>GAMGHKIDTKEDMKILYSEI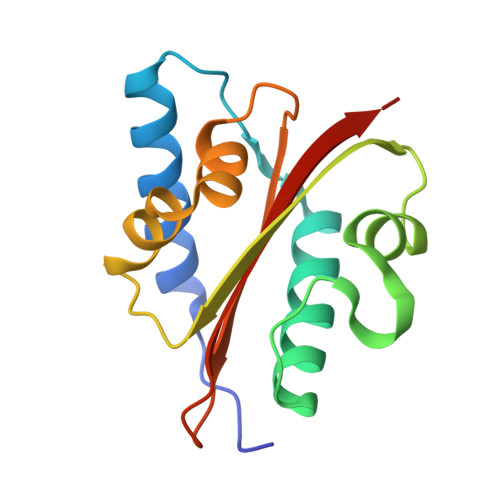AELRKKLNLNHLEIDDTLEKVAKEYAIKLGENRTITHTLFGTTPMQRIHKYDQSFNLTREILASGIELNRVVNAWLNSPSHKEALINTDTDKIGGYRLKTTDNIDIFVVLFGKRKYKN[2x]> MSNYPLHQACMENEFFKVQELLHSKPSLLLQKDQDGRIP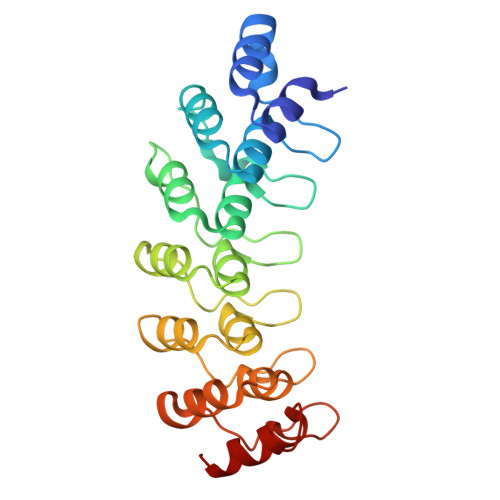LHWSVSFQAHEITSFLLSKMENVNLDDYPDDSGWTPFHIACSVGNLEVVKSLYDRPLKPDLNKITNQGVTCLHLAVGKKWFEVSQFLIENGASVRIKDKFNQIPLHRAASVGSLKLIELLCGLGKSAVNWQDKQGWTPLFHALAEGHGDAAVLLVEKYGAEYDLVDNKGAKAEDVALNEQVKKFFLNNV>[2x]MHKDELLELHEQMVNIKDQFLGFDHVDE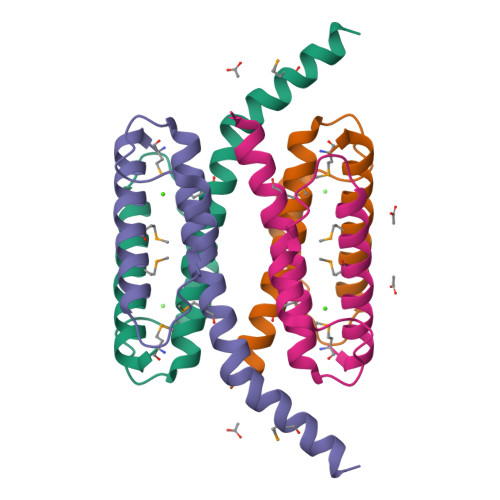TAFAAYEELDVEPSHVHKSKSEHKHAVFLLGNALAAAMSEDEFSSAGRISKRMEELADDASNQLLEHHHHHH> SPSVNQPYRTGFHFQPPKNWMNDPNGPMIYKGIYHLFYQWNPKGAVWGNIVWAHSTSTDLINWDPHPPAIFPSAPFDINGCWSGSATILPNGKPVILYTGIDPKNQQVQNIAEPKNLSDPYLREWKKSPLNPLMAPDAVNGINASSFRDPTTAWLGQDKKWRVIIGSKIHRRGLAITYTSKDFLKWEKSPEPLHYDDGSGMWECPDFFPVTRFGSNGVETSSFGEPNEILKHVLKISLDDTKHDYYTIGTYDRVKDK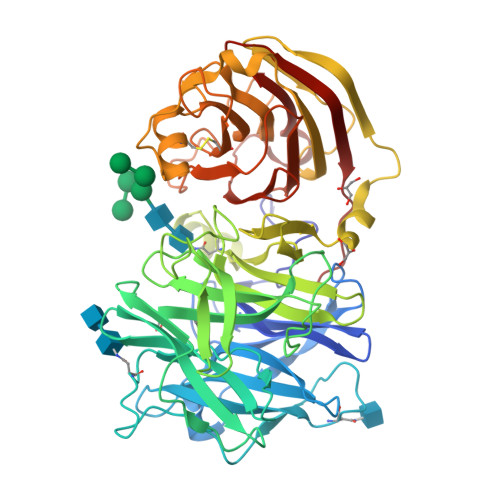FVPDNGFKMDGTAPRYDYGKYYASKTFFDSAKNRRILWGWTNESSSVEDDVEKGWSGIQTIPRKIWLDRSGKQLIQWPVREVERLRTKQVKNLRNKVLKSGSRLEVYGVTAAQADVEVLFKVRDLEKADVIEPSWTDPQLICSKMNVSVKSGLGPFGLMVLASKNLEEYTSVYFRIFKARQNSNKYVVLMCSDQSRSSLKEDNDKTTYGAFVDINPHQPLSLRALIDHSVVESFGGKGRACITSRVYPKLAIGKSSHLFAFNYGYQSVDVLNLNAWSMNSAQIS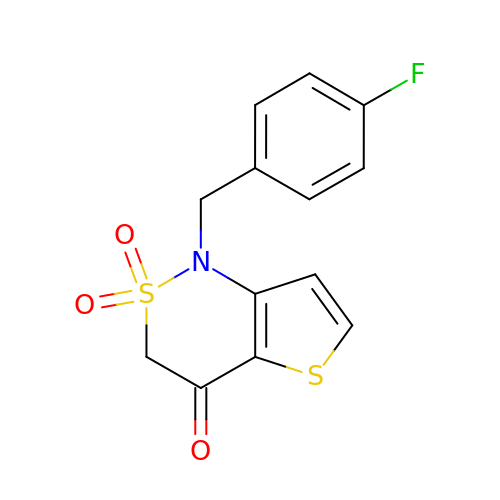1-[(4-fluorophenyl)methyl]-2,2-bis(oxidanylidene)thieno[3,2-c][1,2]thiazin-4-one | C13 H10 F N O3 S2 | CZWDYEYEBHIIQS-UHFFFAOYSA-N> PAQDNSRFVIRDRNWHPKALTPDYKTSIARSPRQALVSIPQS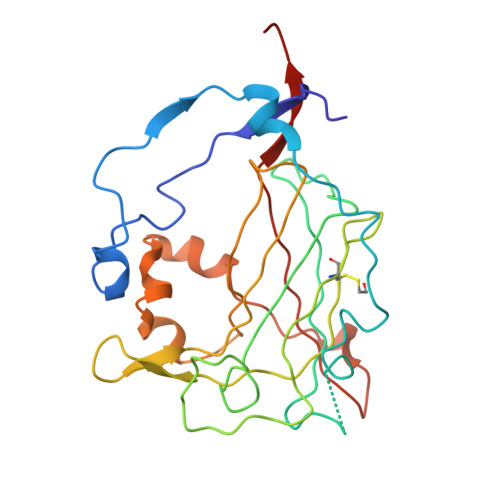ISETTGPNFSHLGFGAHDHDLLLNFNNGGLPIGERIIVAGRVVDQYGKPVPNTLVEMWQANAGGRYRHKNDRYLAPLDPNFGGVGRCLTDSDGYYSFRTIKPGPYPWRNGPNDWRPAHIHFGISGPSIATKLITQLYFEGDPLIPMCPIVKSIANPEAVQQLIAKLDMNNANPMDCLAYRFDIVLRGQRKTHFENC Human cellular retinol binding protein II (hCRBPII) was used as a protein engineering platform to rationally regulate absorptive and emissive properties of a covalently bound fluorogenic dye. We demonstrate the binding of a thio-dapoxyl analog via formation of a protonated imine between an active site lysine residue and the chromophore’s aldehyde. Previously, we showed the utility of human cellular retinol-binding protein II (hCRBPII) mutants as a fluorophoric tag, wherein an active site lysine residue (Q108K) reacts with synthetic aldehydic chromophores, giving rise to the formation of either an imine (Schiff base, SB) or an iminium (protonated SB, PSB). Q108K functions as the active-site lysine and forms a Schiff base with the aldehyde, whereas the K40L mutation is assumed to eliminate interactions between Q108K and Lys40, an interaction that could otherwise impede imine formation, and is also required to promote Schiff base protonation.

Gratifyingly, the red shifting properties of T51V and T53S to M1 were additive, resulting in 47 and 23 nm, absorption and emission red shifts, respectively (M8). Thus, the M8 template (Q108 K:K40L:T51V:T53S) was retained for further protein engineering. We first focused on the Arg58 position, introducing aromatic residues (M9-M12) to the parent tetramutant M8. However, results were disappointing with most mutations resulting in modest hypsochromic wavelength shifts. Additionally, comparison of the M10 and M11 structures shows that introduction of Trp58 results in an almost 90° rotation of the entire chromophore, altering the position and therefore interactions of the imine at the opposite end.

>[2x]TRDQNGTWEMESNENFEGYMKALDIDFATRKIAVRLTQTLVIDQDGDNFKVKSTSTFYNYDVDFTVGVEFDEYTKSLDNRHVKALVTWEGDVLVCVQKGEKENRGWKKWIEGDKLYLELTCGDQVCRQVFKKK> VKLSHVEKDFIAFYSTTPHHLSYRDKTGGSYFITRLISCFRKHACSCHLFDIFLKVQQSFEKA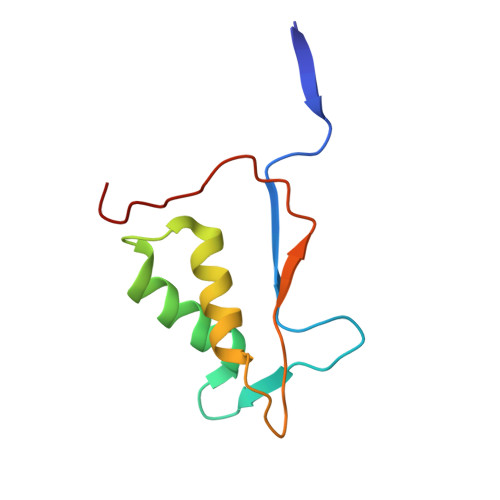SIHSQMPTIDRATLTRYFYLFPGN> MPSSLLGAAMPASTSAAALQEALENAGRLIDRQLQEDRMYPDLSELLMVSAPNNPTVSGMSDMDYPLQGPGLLSVPNLPEISSIRRVPLPPELVEQFGHMQCNCMMGVFPPISRAWLTIDSDIFMWNYEDGGDLAYFDGLSETILAVGLVKPKAGIFQPHVRHLLVLATPVDIVILGLSYANLQTGSGVLNDSLSGGMQLLPDPLYSLPTDNTYLLTITSTDNGRIFLAGKDGCLYEVAYQAEAGWFSQRCRKINHSKSSLSFLVPSLLQFTFSEDDPILQIAIDNSRNILYTRSEKGVIQVYDLGQDGQGMSRVASVSQNAIVSAAGNIARTIDRSVFKPIVQIAVIENSESLDCQLLAVTHAGVRLYFSTCPFRQPLARPNTLTLVHVRLPPGFSASSTVEKPSKVHRALYSKGILLMAASENEDNDILWCVNHDTFPFQKPMMETQMTAGVDGHSWALSAIDELKVDKIITPLNKDHIPITDSPVVVQQHMLPPKKFVLLSAQGSLMFHKLRPVDQLRHLLVSNVGGDGEEIERFFKLHQEDQACATCLILACSTAACDREVSAWATRAFFRYGGEAQMRFPTTLPPPSNVGPILGSPVYSSSPVPSGSPYPNPSFLGTPSHGIQPPAMSTPVCALGNPATQATNMSCVTGPEIVYSGKHNGICIYFSRIMGNIWDASLVVERIFKSGNREITAIESSVPCQLLESVLQELKGLQEFLDRNSQFAGGPLGNPNTTAKVQQRLIGFMRPENGNPQQMQQELQRKFHEAQLSEKISLQAIQQLVRKSYQALALWKLLCEHQFTIIVAELQKELQEQLKITTFKDLVIRDKELTGALIASLINCYIRDNAAVDGISLHLQDICPLLYSTDDAICSKANELLQRSRQVQNKTEKERMLRESLKEYQKISNQVDLSNVCAQYRQVRFYEGVVELSLTAAEKKDPQGLGLHFYKHGEPEEDIVGLQAFQERLNSYKCITDTLQELVNQSKAAPQSPSVPKKPGPPVLSSDPNMLSNEEAGHHFEQMLKLSQRSKDELFSIALYNWLIQVDLADKLLQVASPFLEPHLVRMAKVDQNRVRYMDLLWRYYEKNRSFSNAARVLSRLADMHSTEISLQQRLEYIARAILSAKSSTAISSIAADGEFLHELEEKMEVARIQLQIQETLQRQYSHHSSVQDAVSQLDSELMDITKLYGEFADPFKLAECKLAIIHCAGYSDPILVQTLWQDIIEKELSDSVTLSSSDRMHALSLKIVLLGKIYAGTPRFFPLDFIVQFLEQQVCTLNWDVGFVIQTMNEIGVPLPRLLEVYDQLFKSRDPFWNRMKKPLHLLDCIHVLLIRYVENPSQVLNCE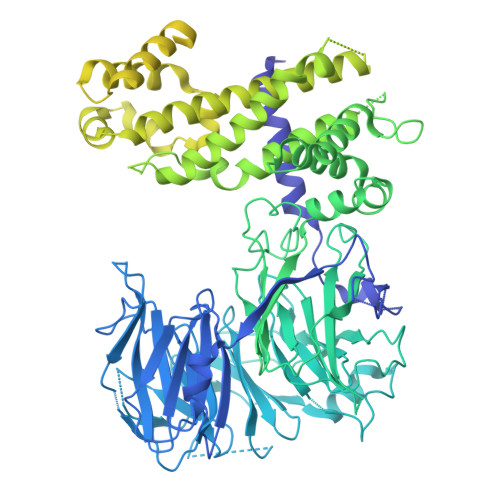RRRFTNLCLDAVCGYLVELQSMSSSVAVQAITGNFKSLQAKLERLH> MGSSHHHHHHGSQQLQNIIETAFERRAEITPANADTVTREAVNQVIALLDSGALRVAEKIDGQWVTHQWLKKAVLLSFRINDNQVIEGAESRYFDKVPMKFADYDEARFQKEGFRVVPPAAVRQGAFIARNTVLM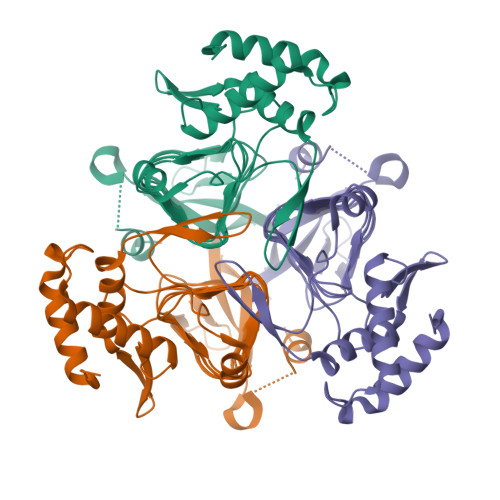PSYVNIGAYVDEGTMVDTWATVGSCAQIGKNVHLSGGVGIGGVLEPLQANPTIIEDNCFIGARSEVVEGVIVEEGSVISMGVYIGQSTRIYDRETGDIHYGRVPAGSVVVSGNLPSKDGKYSLYCAVIVKKVDAKTRGKVGINELLRTID> MCDLRRPAAGGMMDLAYVCEWEKWSKSTHCPSVPLACAWSCRNLIAFTMDLRSDDQDLTRMIHILDTEHPWDLHSIPSEHHEAITCLEWDQSGSRLLSADADGQIKCWSMADHLANSWESSVGSLVEGDPIVALSWLHNGVKLALHVEKSGASSFGEKFSRVKFSPSLTLFGGKPMEGWIAVTVSGLVTVSLLKPSGQVLTSTESLCRLRGRVALADIAFTGGGNIVVATADGSSASPVQFYKVCVSVVSEKCRIDTEILPSLFMRCTTDLNRKDKFPAITHLKFLARDMSEQVLLCASSQTSSIVECWSLRKEGLPVNNIFQQISPVVGDKQPTILKWRILSATNDLDRVSAVALPKLPISLTNTDLKVASDTQFYPGLGLALAFHDGSVHIVHRLSLQTMAVFYSSAAPRPVDEPAMKRPRTAGPAVHLKAMQLSWTSLALVGIDSHGKLSVLRLSPSMGHPLEVGLALRHLLFLLEYCMVTGYDWWDILLHVQPSMVQSLVEKLHEEYTRQTAALQQVLSTRILAMKASLCKLSPCTVTRVCDYHTKLFLIAISSTLK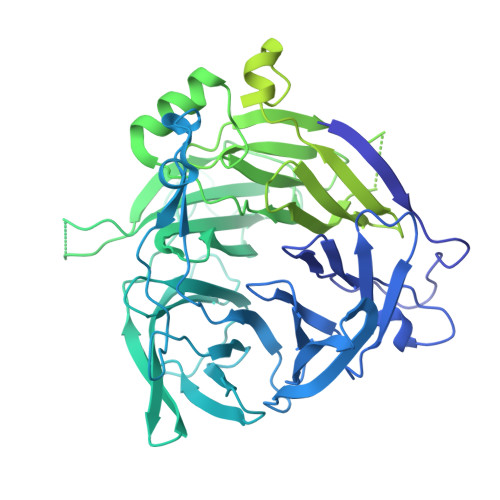SLLRPHFLNTPDKSPGDRLTEICTKITDVDIDKVMINLKTEEFVLDMNTLQALQQLLQWVGDFVLYLLASLPNQGSLLRPGHSFLRDGTSLGMLRELMVVIRIWGLLKPSCLPVYTATSDTQDSMSLLFRLLTKLWICCRDEGPASEPDEALVDECCLLPSQLLIPSLDWLPASDGLVSRLQPKQPLRLQFGRAPTLPGSAATLQLDGLARAPGQPKIDHLRRLHLGACPTEECKACTRCGCVTMLKSPNRTTAVKQWEQRWIKNCLAVEGRGPDACVTSRASEEAPAFVQLGPQSTHHSPRTPRSLDHLHPEDRP> MKIRSPIVSVLGHVDHGKTTLLDHIRGSAVASREAGGITQHIGATEIPMDVIEGICGDFLKKFSIRETLPGLFFIDTPGHEAFTTLRKRGGALADLAILIVDINEGFKPQTQEALNILRMYRTPFVVAANKIDRIHGWRVHEGRPFMETFSKQDIQVQQKLDTKVYELVGKLHEEGFESERFDRVTDFASQVSIIPISAITGEGIPELLTMLMGLAQQYLREQLKIEEDSPARGTILEVKEETGLGMTIDAVIYDGILRKDDTIAMMTSKDVISTRIRSLLKPRPLEEMRESRKKFQKVDEVVAAAGIKIVAPGIDDVMAGSPLRVVTDPEKVREEILSEIEDIKIDTDEAGVVV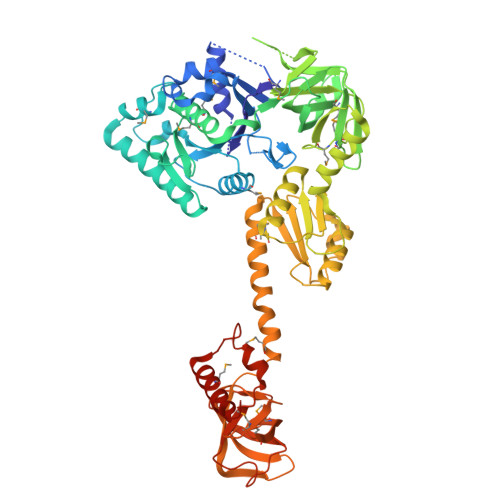KADTLGSLEAVVKILRDMYVPIKVADIGDVSRRDVVNAGIALQEDRVYGAIIAFNVKVIPSAAQELKNSDIKLFQGNVIYRLMEEYEEWVRGIEEEKKKKWMEAIIKPASIRLIPKLVFRQSKPAIGGVEVLTGVIRQGYPLMNDDGETVGTVESMQDKGENLKSASRGQKVAMAIKDAVYGKTIHEGDTLYVDIPENHYHILKEQLSGDLTDEELDLMDKIAEIKRKKNPDWGMKAPF>[2x]HFLCGVVEGFYGRPWVMEQRKELFRRLQKWELNTYLYAPKDDYKHRMFWREMYSVEEAEQLMTLISAAREYEIEFIYAISPGLDITFSNPKEVSTLKRKLDQVSQFGCRSFALLFDNIDHNMCAADKEVFSSFAHAQVSITNEIYQYLGEPETFLFCPTEYCGTFCYPNVSQSPYLRTVGEKLLPGIEVLWTGPKVVSKEIPVESIEEVSKIIKRAPVIWDNIHANDYDQKRLFLGPYKGRSTELIPRLKGVLTNPNCEFEANYVAIHTLATWYKSNMNGVRKDVVMTDSEDSTVSIQIKLENEGSDEDIETDVLYSPQMALKLALTEWLQEFGVPHQYSSRGGGGSGGGGSVTLEDLQLLADLFYLPYEHGPKGAQMLREFQWLRANSSVVSVNCKGKDSEKIEEWRSRAA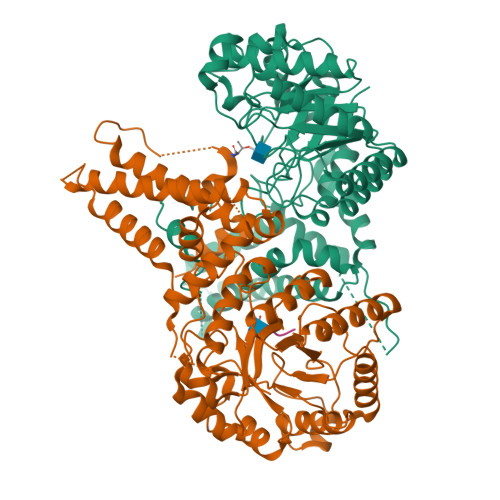KFEEMCGLVMGMFTRLSNCANRTILYDMYSYVWDIKSIMSMVKSFVQWLGCRSHSSAQFLIGDQEPWAFRGGLAGEFQRLLPIDGANDLFFQ;>[2x]FWSTLSPI>[4x]MAKNRRDRNSWGGFSEKTYEWSSEEEEPVKKAGPVQVLIVKDDH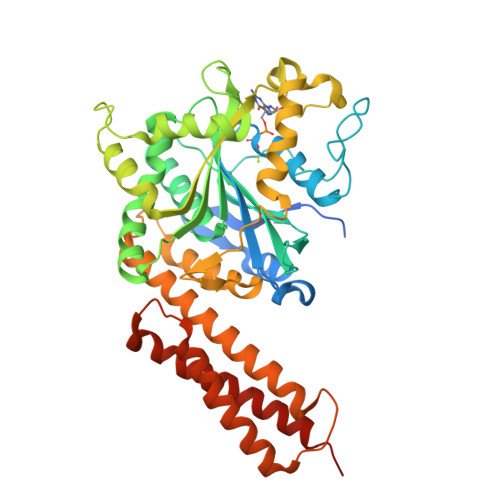SFELDETALNRILLSEAVRDKEVVAVSVAGAFRKGKSFLMDFMLRYMYNQESVDWVGDYNEPLTGFSWRGGSERETTGIQIWSEIFLINKPDGKKVAVLLMDTQGTFDSQSTLRDSATVFALSTMISSIQVYNLSQNVQEDDLQHLQLFTEYGRLAMEETFLKPFQSLIFLVRDWSFPYEFSYGADGGAKFLEKRLKVSGNQHEELQNVRKHIHSCFTNISCFLLPHPGLKVATNPNFDGKLKEIDDEFIKNLKILIPWLLSPESLDIKEINGNKITCRGLVEYFKAYIKIYQGEELPHPKSMLQATAEANNLAAVATAKDTYNKKMEEICGGDKPFLAPNDLQTKHLQLKEESVKLFRGVKKMGGEEFSRRYLQQLESEIDELYIQYIKHNDSKNIFHAART>[2x]MTRRTAFFFDELCLWHAAGPHALTLPVGGWVQPPAAAGHAESPETKRRLKSLLDVSGLTARLQLRSAPPASDEDLLRVHPAHYLERFKALSDAGGGSLGQDAPIGPGSYEIARLSAGLAIAALDAVLAGEADNAYSLSRPPGHHCLPDQAMGFCFFANIAVAIEAAKARHGVERVAVLDWDVHHGNGTQAIYYRRDDVLSISLHQDG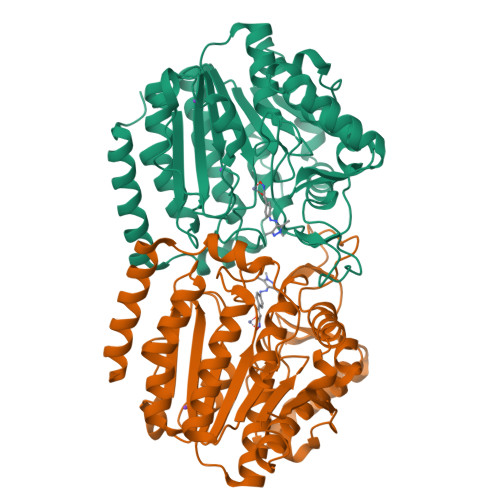CFPPGYSGAEDIGEDRGRGFNLNVPLLPGGGHDAYMQAMQRIVLPALERFRPQLIVVASGFDANAVDPLARMQLHSDSFRAMTAMVRDAAERHAGGRLVVVHEGGYSEAYVPFCGLAVIEELSGVRSAVRDPLRDFIELQQPNAAFRDFQRQRLEELAAQFGLCPAQPLQAAR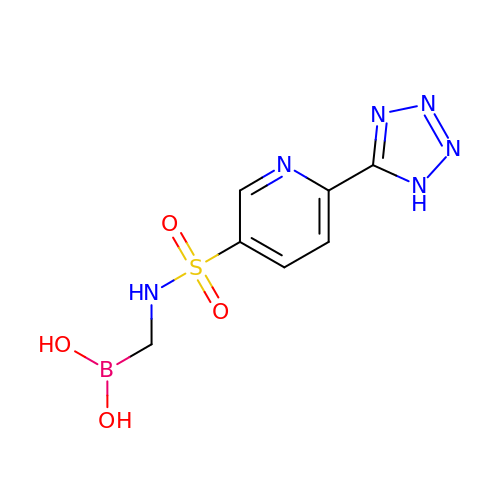[({[6-(1H-tetrazol-5-yl)pyridin-3-yl]sulfonyl}amino)methyl]boronic acid | C7 H9 B N6 O4 S | HHNYNQPNDNBATH-UHFFFAOYSA-N> MPLELTQSRVQKIWVPVDHRPSLPRSCGPKLTNSPTVIVMVGLPARGKTYISKKLTRYLNWIGVPTKVFNVGEYRREAVKQYSSYNFFRPDNEEAMKVRKQCALAALRDVKSYLAKEGGQIAVFDATNTTRERRHMILHFAKENDFKAFFIESVCDDPTVVASNIMEVKISSPDYKDCNSAEAMDDFMKRISCYEASYQPLDPDKCDRDLSLIKVIDVGRRFLVNRVQDHIQSRIVYYLMNIHVQPRTIYLCRHGENEHNLQGRIGGDSGLSSRGKKFASALSKFVEEQNLKDLRVWTSQLKSTIQTAEALRLPYEQWKALNEIDAGVCEELTYEEIRDTYPEEYALREQDKYYYRYPTGESYQDLVQRLEPVIMELERQENVLVICHQAVLRCLL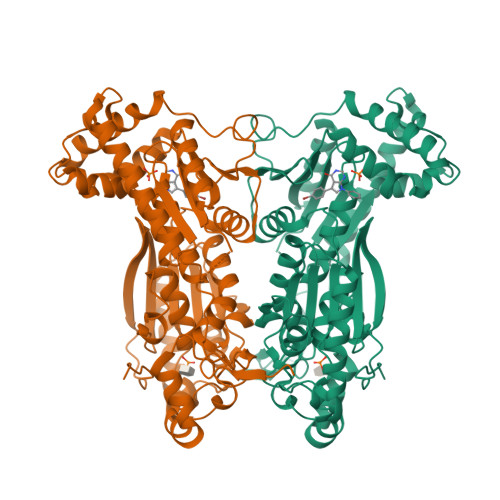AYFLDKSAEEMPYLKCPLHTVLKLTPVAYGCRVESIYLNVESVCTHRERSEDA N-{(5E)-10-[(9E)-tetradec-9-enoylamino]dec-5-enoyl}-L-seryl-N-(2-cyclohexylethyl)-L-lysinamide 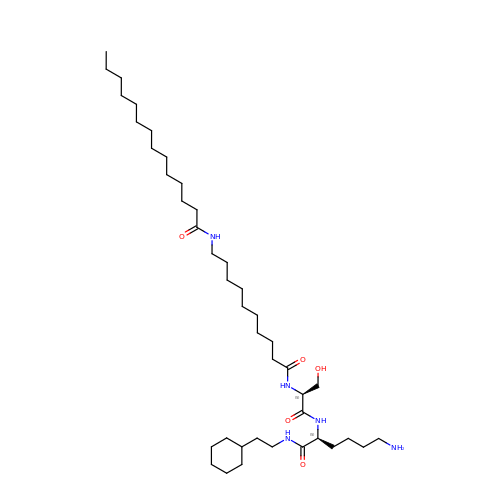| C41 H79 N5 O5 | QIQBRVNLNJERKS-FBKDKWTRSA-N>GSHMELTPDQQTLLHFIMDSYNKQRMPQEITNKIL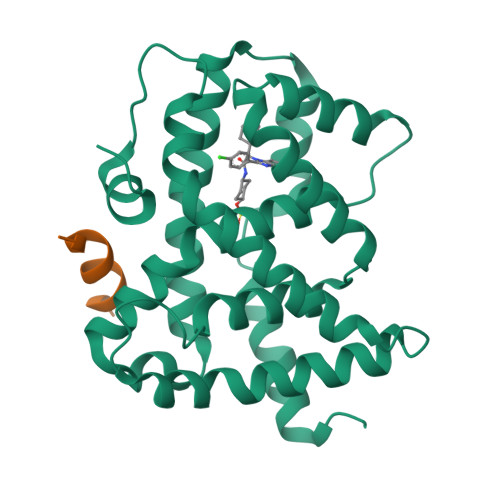KEAFSAEENFLILTEMATNHVQVLVEFTKKLPGFQTLDHEDQIALLKGSAVEAMFLRSAEIFNKKLPSGHSDLLEARIRNSGISDEYITPMFSFYKSIGELKMTQEEYALLTAIVILSPDRQYIKDREAVEKLQEPLLDVLQKLCKIHQPENPQHFACLLGRLTELRTFNHHHAEMLMSWRVNDHKFTPLLCEIWDVQ[2x];>[2x]KDHQLLRYLLDKDE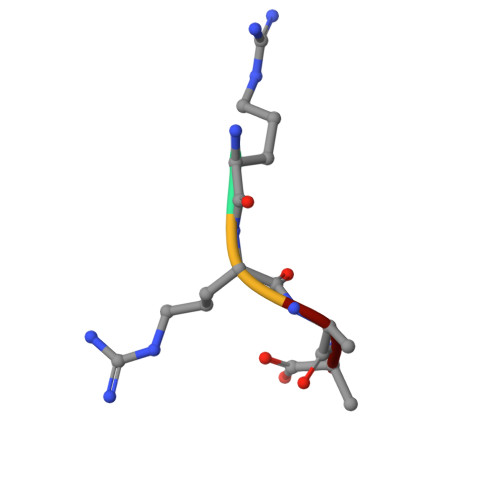> RRAA The mitochondrial ATP synthase is a membrane protein complex that generates most of the ATP in eukaryotic cells. The translocation of protons through the membrane-bound Fo part, mediated by subunit a, drives the rotation of a membrane-embedded c-ring and the attached central stalk, which together form the rotor. The torque of the rotor against the stator subunits induces conformational changes in the (αβ)3 headpiece, thereby triggering catalysis. To reveal how the mitochondrial ATP synthase is modulated by lipids and organised into a dimer shaping discoid cristae in Euglenozoan mitochondria, we determined the structure of the ATP synthase dimer from E. gracilis.

Symmetry expansion of the pseudo-C2-symmetric dimer particles was used to classify individual F1/c-ring monomers into rotational states 1, 2 and 3 (named according to bovine nomenclature; Zhou et al., 2015) and resolve structures at 3.0- to 3.9 Å resolution. The E. gracilis F1/cring maps of rotational states 1 and 2 showed strong density for IF1, but weak density in rotational state 3. Subsequent focused classification of the IF1 binding site suggested complete inhibitor binding for rotational states 1 and 2, whereas rotational state 3 displayed a mixed occupancy, with a minority (34%) of particles containing IF1 and a majority (66%) not containing the inhibitor. Unlike the bovine ATP synthase, which displays a nearly equal particle distribution among the three rotational states, rotational state-3 (20%) is less populated than rotational states 1 (44%) and 2 (36%). Rather than reflecting dwell times during rotary catalysis, the distribution of rotational states is likely dictated by accessibility of the respective catalytic interfaces to IF1 binding, which for rotational state-3 may be sterically hindered by the proximity to the peripheral stalk. In all three rotational states, IF1 is bound to the βDP-αDP interface adopting a similar conformation. We observe this contact in all three rotational states, which provides the first observation of an interaction between the peripheral and central stalk in the ATP synthase. The position of the lumenal H5EG1 on the c-ring β-barrel remains largely unchanged in all three rotational states, suggesting a mechanism of transient rotor-stator interaction during c-ring rotation.

>MHYAEAATPAKSAGSAVAKKHLEAKQKIGFVHGIDGTIATIAPAASKVTVPYNTVLEIAVSATNIANALVFNLEKDGSIGVILLDNISEVRSGQDVYATGSLLKIPVGFHMLGKIINPLGKEIPTGLFTKAAPLLDDTKLGLVEEMAPNIVSRQPVNYNLLTGYKVIDTLIPVGRGQRELILGDRQTGKTSIALSTILNQTKVNNEILSKNNVLSVYVSIGQRCSNVARIHRLLTEYDAMKYCTIVAATAADPAGLQYLAPYAGTTLGEEFRNSGRHILLVYDDLSKQAVSYRQISLLLRRPPGREAYPGDVFYLHSRLLERSAMMSPQKGSGSLTSLPIVETLSNDVTAYIVTNVISITDGQIYLDAKLFTGGQRPAVNIGLSVSRVGSSAQNKAMKKVGGALKMLMGEYRKMAGEQTSGSQNVSPVMIRGARCLQLFNQKGPSYFMDAIVALYAVTNGYMDDVKLQYSKFYEFLLLNKDLPVLYGQVNNKYFYMYNKNLNYFIRYFGLNHEILEPELKKYIEIHTNLFLDNYQSRMNELKSDEDLVQLKNLLYACKRTV[3x];>[3x]TAPATAADVKQVGYVQQIIGAVVDVTFTDSVPPVLTALTVDAKETGTLLTMEIVQHLDTKTARCICMSSTDMLRLRTPVVNTGSQITVPVGEATLGRIFNVMGDAIDQRGPVKNKVRWPIHRKAPTLAEQSGKDEVLVTGIKVIDLILPYCKGGKIGLFGGAGVGKTVIIMELINNVAKGHGGYSVFAGVGERTREGTDLYLEMMGSKVIDLQGDSKCVLVYGQMNEPPGARARVAQTALTMAEYFRDEAGQDVLLFVDNVFRFTQANSEVSALLGRIPAAVGYQPTLAEDLGMLQERITSTVKGSITSVQAVYVPADDITDPAPATTFSHLDATTVLSRSVAEAGIYPAVEPLECASRIMDPDAIDVNHYNVAMDIVEMLTKYKELQDIIAVLGIDELSEEDKLIVDRARKVAKFMSQPFAVAEVFTGMKGYYVQLEDCVSDFGSLLMGQCDNIPEMAFYMVGGLDSVKEKAAKMAAEAAAMRERARKAAEAK;> MPGGGTIRFWREKLEGYKKYHQIVKTIKMVTLAKYRQTVVRTRVRDQTLRYTRKALDAKTQDDQEVIEKSECLLYVPITTNRGSCGALNTNMVRYLQEVENPKMTIISVGKKALDAMTKVFQDTYRRTILNDMKQAMSFQFAAYVLEHMNTVPWDRAQIVYNRYHGAASQKLAIFNLPKFEDWKQKLEEDSAGDGKIEEDGLLQSLPMKTALGELEETAVEDFYNFHSCLAVLNAVSENELSEYAARIVAVENQLGNITGLMQLADYTYNKTRKELITAELLEIIGTMTAMHAGKKVGLKKTEFWK;> MRASRTLLLSVSRFMRQDPRKFFPDNGFRFFDGPEDSFGDGNIPAQIILTLTRQDEFILKQEPVAAITIRTNEGEMGVLAGHEYTVQQLAPGILEVEYEGGKKDQYVISGGFAHVNDTGVVDINTVEAVPLEEIDHEKLAKALEEARAKSQSPDEAVRIQGEIALEIFEPLEAALH;> MSWRDAGISYLRYLSIVTRCIHEVQKEGPLLTKNVRFSTIGWKSLYLDHGATKEYTAIPAELEKIPENQVAQQHHA;>MQKLSRVVCNRLVRFHGTVAASAGGKRYDLFGYEVSVATGPFIEEIKKAQFYDDAGEVIVKMNLANTPPDLQTYNAVLERILNCKSKRSQPVKGENKFAAMMDILEEMDARSGIKPNAESWGYVLKELVQAGDFRLGWVCIAGMKSLGITPDQALVDANEANAAKAKAAGTDFPAYLKKAAPESFDTKAWGI[3x];> MHMRRAVSVFGRCRSLNGLRNYAVPSPKYIEIYQSDFSRNAYPLELLGGSHVDFAKLLYSFADQVENKKFEVYVEDFKKLDSIIAEKGPFWAEEKIFQSPTFQGLSEGFKFILGWIQSEGAIDRLENVRLAYKELVNEARKETTATVIVAKEPSGNDLAEIRKQVEELHKESPLKDYKLVLETKVDPSIGGGYILEVCNQVVNRSAAAAAAETAALAKASAAQVDWTSLPAAPPRPSPSAPDTLIRLLGSVVDDLADADKVEQKYGA;> MAAACAVRGFTTARPMLTPNKVKVPGRKPQDEEDLTWAEADRKLTPEERYARDKQMALLDKMTSQVEELEKSHTEQKKSNKGVKAQIEAISRQLEALKAQLKE;>[10x]MQRGSSITKVVRRAALARSTRNAAIAYEVTVNGANLIGAGMAASGVGVPAIGVAMCFSSYMLAAARQPNMSAKLLPYCILGFALSEALALFTLLIALLELFVFS;> MFRGFRPVLAADAVKFQTLYNVLTGKQHLKDQVPVKDCNLTAIFGASWKADLNKWFDSEYAPKLPAAERDSAKKSLDLYLKRVDLTRYTREELTTYGILACGPGKVDALTEKHLLETGKARLEELTAGLGNKDEGVNAFRKEVEQEGKYANWPAEKSKALADKVIAASP;> MMRRACRIIRPSHVRGVSGVAPTIYLRSKAALPATSTTDVRPQLYALQRFAKAQLKTATEAERAAIEADIARYQEYLDSDLEKLKQDVAEDTAKKQKLIPLLDRYPDVPIEKIPEHANVLLKKIDACLEILSKDIGEVTDAEAHEMYFETSKFQILHIYTGCVASFPEGDVPPGAVECLPGQVIRTKVNGEDVMLEIDEVDPGYQVCWFKPDVPLPENAEILWSYPYEPTAALPTGTTWEEGQANVLIPAEPTPEAAVWPPTPVTNVYAPMAEKLALKSNPELKVLFKEALLQPAKLLPLDVDYQCSHDREVVEAKRDRYLTALVEAEQAPPLPFTPDVLQLQLEHNVLKGELIDRLRALEYTIVTEQLQARLHERRLRGDVIDEWEELDYHPLVRDDTYLAIDFGDPTFGRYIWKLFPHTDGDEECMFKDTRLDVLPPQVNPLNAILAQHTAQTPVHRSLEKRLWTEVRATAVSE> SATSTTIAKHIGNSNPLIDHHLGADPVALTYNGRVYIYMSSDDYEYNSNGTIKDNSFANLNRVFVISSADMVNWTDHGAIPVAGANGANGGRGIAKWAGASWAPSIAVKKINGKDKFFLYFANSGGGIGVLTADSPIGPWTDPIGKPLVTPSTPGMSGVVWLFDPAVFVDDDGTGYLYAGGGVPGVSNPTQGQWANPKTARVIKLGPDMTSVVGSASTIDAPFMFEDSGLHKYNGTYYYSYCINFGGTHPADKPPGEIGYMTSSSPMGPFTYRGHFLKNPGAFFGGGGNNHHAVFNFKNEWYVVYHAQTVSSALFGAGKGYRSPHINKLVHNADGSIQEVAANYAGVTQISNLNPYNRVEAETFAWNGRILTEKSTAPGGPVNNQHVTSIQNGDWIAVGNADFGAGGARSFKANVASTLGGKIEVRLDSADGKLVGTLNVPSTGGAQTWRE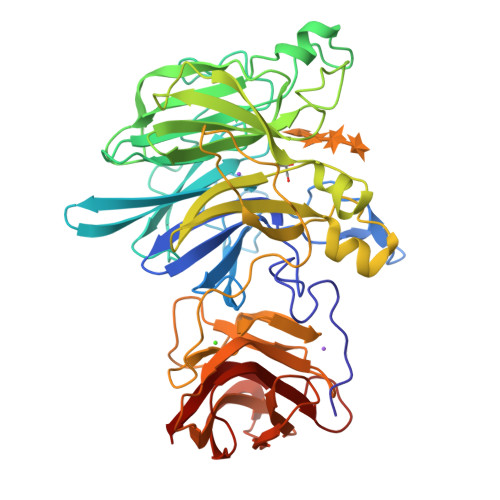IETAVSGATGVHKVFFVFTGTGTGNLFNFDYWQFTQR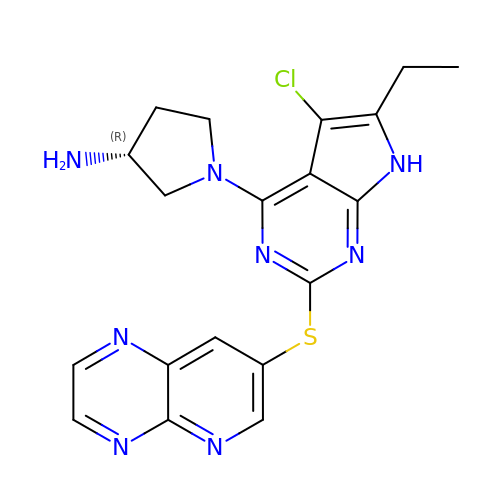(3R)-1-[5-chloro-6-ethyl-2-(pyrido[2,3-b]pyrazin-7-ylsulfanyl)-7H-pyrrolo[2,3-d]pyrimidin-4-yl]pyrrolidin-3-amine | C19 H19 Cl N8 S | WXCUMDKJRMUULE-SNVBAGLBSA-N>GUAXGUAC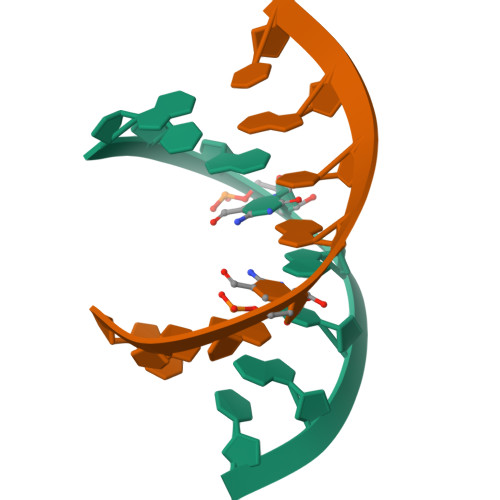[13x]7-{7-[(1R)-1-{[(4P)-6-amino-3H-purin-3-yl]methyl}-5-hydroxy-8-methyl-1,6-dihydropyrrolo[3,2-e]indole-3(2H)-carbonyl]-4-hydroxy-5-methoxy-1,6-dihydropyrrolo[3,2-e]indole-3(2H)-carbonyl}-4-hydroxy-5-methoxy-1,6-dihydropyrrolo[3,2-e]indole-3(2H)-carboxamide 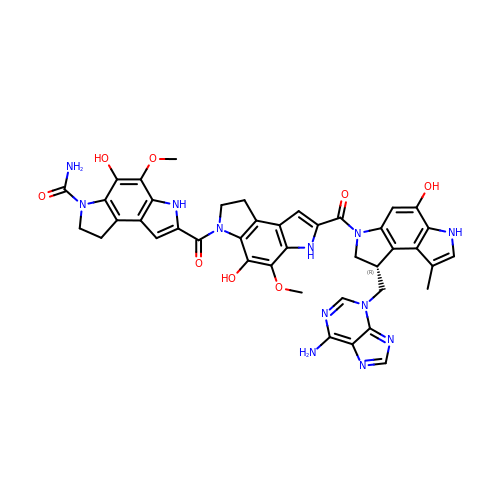| C42 H38 N12 O8 | NZVDCTGEHMJZMN-QGZVFWFLSA-N>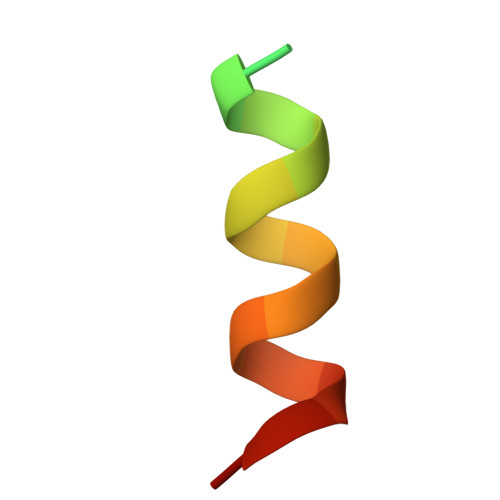 DPTPSDNPFSKLYKETIETFD> GUGTACA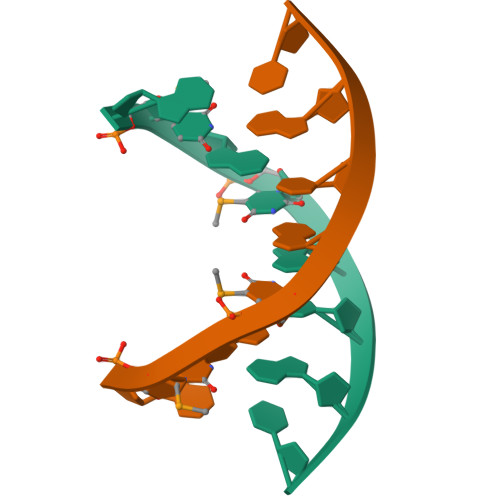C~{N}-[3-acetamido-5-[(5-ethanoyl-2-ethoxy-phenyl)carbamoyl]phenyl]furan-2-carboxamide 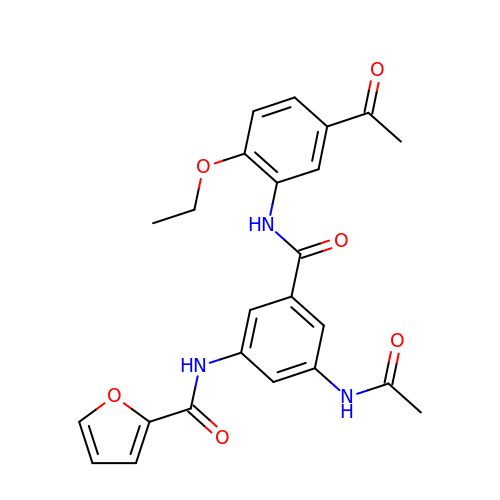| C24 H23 N3 O6 | CERSGKCXWDUOHE-UHFFFAOYSA-N> SVLELGKMILQETGKNAITSYGSYGCNCGWGHRGQPKDATDRCCFVHKCCYKKLTDCNHKTDRYSYSWKNKAIICEEKNPCLKEMCECDKAV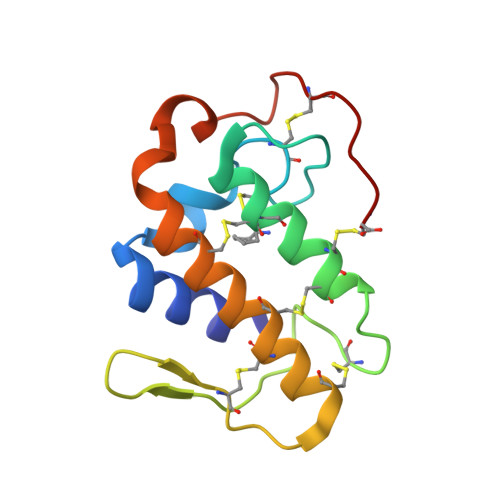AICLRENLDTYNKKYKAYFKLKCKKPDTC> GAGCAGACCTG;> ACACCACTCA;> CATGT;> TCTGAGTGGGGTCTGC

In this work, we exhaustively probe the ability of all 36 immobile HJ sequences to form DNA crystals in two different designed systems. Three separate self-assembling DNA crystal systems are described in this report: the “4 × 5” and “4 × 6” designs (collectively referred to as the 4 × N systems), and a third construct with a “scrambled” sequence variant of the 4 × 6 lattices. Self-assembly was mediated by three constituent oligonucleotides: (S1) containing four sequence repeats of either 5 or 6 bases; (S2) composed of 21 bases containing complementary regions to both (S1); and (S3) which forms the second junction crossover. The HJ serves as the fundamental component at the core of each unit, and the ultimate assembly of the full lattice is facilitated by the complementary 2-base sticky ends that tail each duplex.

The 4 × 5 system robustly crystallized with 75% of the junctions, and we obtained crystals in all but 9 of 36 sequences. Of the resulting structures, 18 exhibited P32 symmetry with average cell dimensions a = b = 68.85 Å c = 60.09 Å, with only nine retaining the original P3221 symmetry with average cell edges a = b = 68.17 Å c = 60.60 Å. Although the cell parameters between the two symmetries were virtually indistinguishable, the differences between the periodicity of the lattices is dramatic, with vastly different cavity sizes. While the highest resolution achieved for the J1 system was 3.1 Å, in roughly half of the crystals measured the resolutions were 3.05 Å or better, and as high as 2.9 Å (J6) and 2.75 Å (J19), for the P32 and P3221 symmetries, respectively. Pos1 and 2 were readily observable in the electron density maps at either one or both of these conserved sites in a significant number of the structures, with no apparent respect to motif or symmetry. However, in the majority of the crystal structures reported here, the cacodylate anion indeed fits best into the electron density map of our X-ray structures, due to the presence of sodium cacodylate in the crystallization solution.> AYVEIIEQPKQRGMRFRYKCEGRSAGSIPGERSTDTTKTHPTIKINGYTGPGTVRISLVTKDPPHRPHPHELVGKDCRDGYYEADLCPDRSIHSFQNLGIQCVKKRDLEQAISQRIQTNNNPFHVPIEEQRGDYDLNAVRLCFQVTVRDPAGRPLLLTPVLSHPIFDNRA;> GAMSHPHDSKVFPDLPEHQDNPSQLRLQHDGLATDDKARLEPMCLAEYLISGPGGMDPDIEIDDDTYDECREVLSRILEDAYTQSGTFRRLMNYAYDQELHDVEQRWLLGAGENFGTTVTDEDLESSEGRKVIALNLDDTDDDSIPEYYESNDGPQQFDTTRSFIHQVVHALTHLQDKEDSNPRGPVVEYTNIILKEMGHTSPPRIAYEFSN

Here, we report that the zinc metalloprotease T3SS effector proteins GtgA, GogA, and PipA from S. enterica cleave a subset of NF-κB subunits comprising p65, RelB, and cRel, whereas NleC from EPEC/EHEC cleaves all five NF-κB subunits. GtgA, in both its apo-form and in complex with p65, has a globular structure, with the catalytic core assuming a Zincin-like fold. The active-site helix (αG) sits at the bottom of a cleft formed between an upper NSD and a lower CSD. Similar to NleC, the active-site cleft of GtgA is highly negatively charged, and the active-site cleft mimics the shape of the DNA major groove.

To prevent cleavage of p65 by GtgA during crystallization, GtgA was inactivated by mutating the glutamate residue in the HEXXH motif to a glutamine (E183Q). GtgA(20–228)E183Q–p65(20–188) crystals belong to space group P212121 with a single heterodimer in the asymmetric unit (a.u.). Residues 20–27 and 137–145 and the C-terminal residue Asn-228 are not visible in the electron density of GtgA(20–228)E183Q nor are the two C-terminal residues of p65(20–188) (residues Arg-187 and Ala-188). GtgA interacts with the p65 NTD via a large interface with a buried surface area of 1081 Å2. Most of the residues in p65 that interact with GtgA, including the p65 cleavage site, are in the loop connecting strands β1′ and β2′, with secondary binding interactions represented by the positively charged surface of the loop connecting strand β7′ and helix αA′ in p65 and the negatively charged surface of the loop connecting helices αC and αD in GtgA. The αF helical segment present in the GtgA apo structure is invisible in the electron density of the GtgA–p65 complex. Despite the absence of the active-site zinc atom in the complex structure of GtgA–p65, the carbonyl oxygen of the P1 residue Gly-40 is positioned above the zinc-coordinating site, hydrogen-bonded with GtgA His-182 and Asp-193. The P1′ residue Arg-41 inserts into the negatively charged S1′ pocket formed by the N-terminal portion of the upper rim and the right wall of the active-site cleft. The side chain of p65 Arg-41 is sandwiched by hydrophobic contacts in between the aromatic rings of Phe-131 and Phe-174, with its guanidino group directly hydrogen-bonded to the side chains of GtgA Asp-155, Glu-163, and Ser-179. Within the active-site cleft of GtgA, the backbone of p65 Glu-39 is hydrogen-bonded to the backbone of Thr-133 of GtgA, whereas its side chain forms hydrogen bonds with the side chains of GtgA residues Gln-192 and Asp-193.5-(2,6-dimethylphenyl)thiophene-2-carboxylic 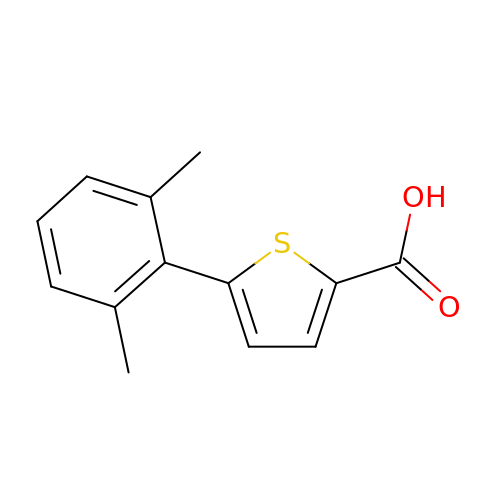acid | C13 H12 O2 S | OIKZRFRQYNLPMK-UHFFFAOYSA-N>[2x]SQNVSLRELAEKLNIYIGFA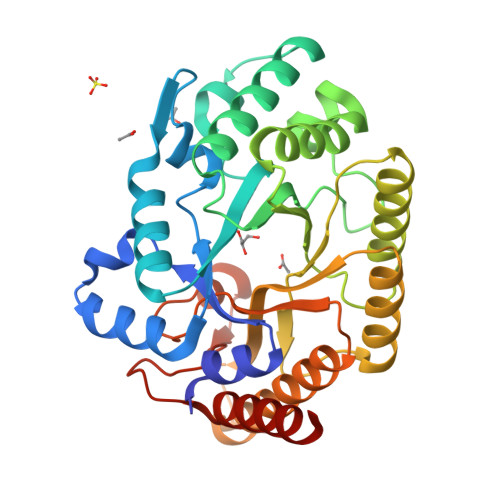AINNFWSLSDAEKYMEVARREFNILTPENQMKWDTIHPERDRYNFTPAEKHVEFAEENDMIVHGHTLVWHNQLPGWITGREWTKEELLNVLEDHIKTVVSHFKGRVKIWDVVNEAVSDSGTYRESVWYKTIGPEYIEKAFRWAKEADPDAILIYNDYSIEEINAKSNFVYNMIKELKEKGVPVDGIGFQMHIDYRGLNYDSFRRNLERFAKLGLQIYITEMDVRIPLSGSEEYYLKKQAEVCAKIFDICLDNPAVKAIQFWGFTDKYSWVPGFFKGYGKALLFDENYNPKPCYYAIKEVLEKKIEERK Unlike SETD3 or METTL18, which methylates a unique substrate, METTL9 specifically recognizes an xHxH motif (H is for histidine and x denotes small residues.) and catalyzes the methylation of the second histidine. xHxH, as a known metal binding motif, is found in a wide range of metal binding proteins, suggesting the potential role of METTL9-dependent histidine methylation in mediating the metal binding capacities for those proteins. Based on the predicted METTL9 structure from AlphaFold11, we chose to mutate its surface-exposed hydrophobic residues to stabilize the protein. One METTL9 fragment (METTL946–318) with six mutations, named METTL9M6 afterwards, exhibited high solubility and homogeneity. In all METTL9M6 complexes, H1 and H-2 are snugly positioned into histidine-specific pockets, while x-1 forms hydrogen bond or hydrophobic interactions with METTL9M6 and x-3 stacks with the aromatic ring of METTL9M6 Tyr306.

To understand the selectivity of METTL9 toward residues at the −1 position, we further solved the structure of METTL9M6 with the SLC39A5 mutant S374A (S-1A) at a resolution of 2.75 Å with the mutant peptide well resolved. In the structure, Ala374 (“A-1”) forms hydrophobic interactions with Met126 and Cys297 of METTL9M6, with a distance of 3.8 Å between Ala374 and the main chain carbonyl group of METTL9M6 Gly124. Any residue at the −1 position larger than Ser or Ala is disfavored because of potential steric clash with the main chain of Gly124.

>[2x]HMAAGGRKENHQWYVCNREKLCESLQAVFVQSYLDQGTQIFLNNSIEKSGWAAIQAYHSAVSSAFSLAMSRTSINGLLGRGSMFVFSPDQFQRLLKINPDWKTHRLLDLGAGDGEVTKIMSPHFEEIYATELSETMIWQLQKKKYRVLGINEWQNTGFQYDVISCLNLLDRCDQPLTLLKDIRSVLEPTRGRVILALVLPFHPYVENVGGKWEKPSEILEIKGQNWEEQVNSLPEVFRKAGFVIEAFTRLPYLCEGDMYNDYYVLDDAVFVLKPV;>[2x]GHQGHAHGHQGG> KENALL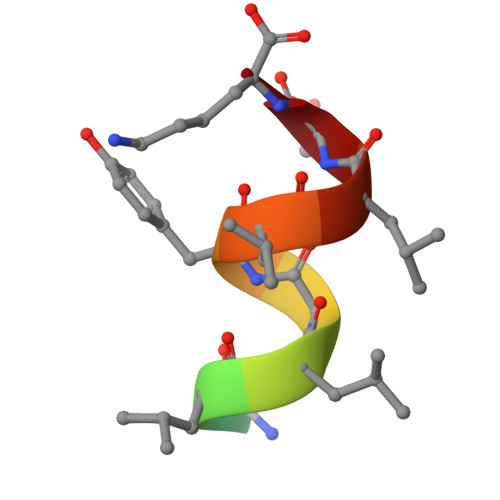RYLLDK> MGSDKIHHHHHHMKEIDELTIKEYGVDSRILMERAGISVVLAMEEELGNLSDYRFLVLCGGGNNGGDGFVVARNLLGVVKDVLVVFLGKKKTPDCEYNYGLYKKFGGKVVEQFEPSILNEFDVVVDAIFGTGLRGEITGEYAEIINLVNKSGKVVVSVDVPSGIDSNTGKVLRTAVKADLTVTFGVPKIGHILFPGRDLTGKLKVANIGHPVHLINSINRYVITREMVRSLLPERPRDSHKGTYGKVLIIAGSRLYSGAPVLSGMGSLKVGTGLVKLAVPFPQNLIATSRFPELISVPIDTEKGFFSLQNLQECLELSKDVDVVAIGPGLGNNEHVREFVNEFLKTLEKPAVIDADAINVLDTSVLKERKSPAVLTPHPGEMARLVKKTVGDVKYNYELAEEFAKENDCVLVLKSATTIVTDGEKTLFNITGNTGLSKGGSGDVLTGMIAGFIAQGLSPLEASTVSVY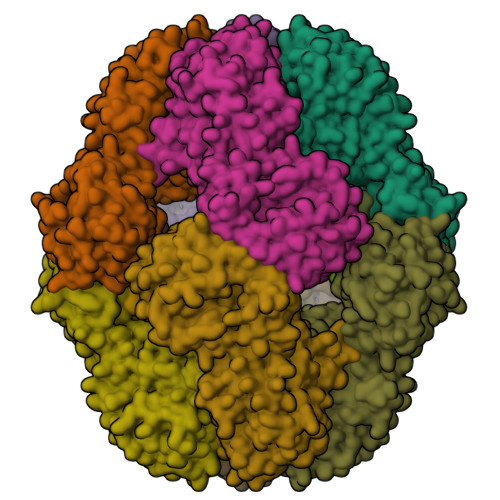LHGFAAELFEQDERGLTASELLRLIPEAIRRLKE;> APAWLFEA> GSTEVQKNQVLTLEEWQDKWVNGKTAF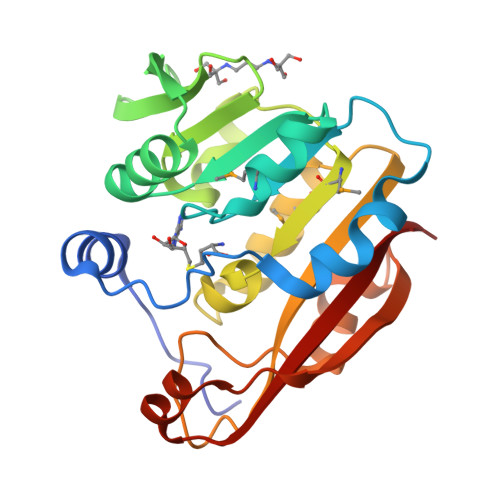HQEQGHQLLKKHLDTFLKGKSGLRVFFPLCGKAVEMKWFADRGHSVVGVEISELGIQEFFTEQNLSYSEEPITEIPGTKVFKSSSGNISLYCCSIFDLPRTNIGKFDMIWDRGALVAINPGDRKCYADTMFSLLGKKFQYLLCVLSYDPTKHPGPPFYVPHAEIERLFGKICNIRCLEKVDAFEERHKSWGIDCLFEKLYLLTEK>[2x]APLHIDTALPDAAQIQQSNSWLEISLGQFQSNIEQFKSHMNANTKICAIMKADAYGNGIRGLMPTIIAQGIPCVGVASNAEARAVRESGFKGELIRVRSASLSEMSSALDLNIEELIGTHQQALDLAELAKQSGKTLKVHIALNDGGMGRNGIDMTTEAGKKEAVSIATQPSLSVVGIMTHFPNYNADEVRAKLAQFKESSTWLMQQANLKREEITLHVANSYTALNVPEAQLDMVRPGGVLFGDLPTNPEYPSIVSFKTRVSSLHHLPKDSTVGYDSTFTTSRDSVLANLPVGYSDGYPRKMGNKAEVLINGQRAKVVGVTSMNTTVVDVTEIKGVLPGQEVVLFGQQQKQSIAVSEMENNAELIFPELYTLWGTSNPRFYVKENLYFQ

Interestingly, V. cholerae encodes an additional multispecific amino acid racemase, named BsrV for broad-spectrum racemase Vibrio, which produces non-canonical DAAs (NCDAAs), i.e., DAAs that are different from those usually present in the cell wall. As Ala-R, BsrV uses pyridoxal 5-phosphate (PLP) as a cofactor and can efficiently racemize Ala. However, BsrV produces nine additional DAAs, including the non-β-branching aliphatic amino acids (Leu, Met, Ser, Cys, Gln and Asn) and the positively charged amino acids (His, Lys and Arg). In this context, BsrV is expressed, and its activity drives the production and release of millimolar concentrations of NCDAAs to the extracellular media.

In a previous study, we reported the three-dimensional structure of BsrV and defined a molecular fingerprint of conserved residues that define the family of broad-spectrum racemases. Compared to Ala-R, BsrV’s capacity to accommodate amino acid substrates other than Ala capitalizes on its broader entry channel and active site. We discovered that contrary to Vibrio cholerae alanine racemase AlrV highly compacted active site, BsrV’s is broader and can be occupied by cell wall stem peptides. Using a BsrV-His variant, we observed that the hexahistidine affinity tag was fully stabilized in BsrV’s entry channel. Based on these data, we proposed that BsrV might interact with the cell wall muropeptides. Using in vitro biochemical and structural analyses, we demonstrated that peptidoglycan peptide moieties bind and inhibit BsrV activity. Interestingly, edited muropeptides containing NCDAAs (produced by BsrV) showed stronger binding and inhibitory properties compared to those ending in D-Ala (canonical muropeptides), suggesting that BsrV activity is controlled via a negative feedback loop by the degree of NCDAA cell wall editing. Taking these biochemical and structural data together, we propose that inhibition of BsrV by peptidoglycan peptides underlies a negative regulatory mechanism to avoid excessive NCDAA production.Mediator of ERBB2-driven cell motility 1 (MEMO1) is an evolutionary conserved protein implicated in many biological processes; however, its primary molecular function remains unknown. MEMO1 is a highly conserved protein found in the cytosol of eukaryotic cells from yeast to humans. We conclude that MEMO1 is an iron-binding protein that modulates iron homeostasis in cancer cells. Our work reveals that the iron coordination mode in MEMO1 is very similar to that of iron-containing extradiol dioxygenases, which also display a similar structural fold.

To confirm the iron-binding site, we generated H49A and C244S mutants, along with H192A and D189N variants, because the latter residues are located in the proximity of the bound iron and were previously proposed to belong to the metal-binding site of the protein. All the mutant proteins were properly folded as shown by NMR. As shown by ITC, iron-binding affinity in the H192A and D189N mutants is not significantly changed, whereas H49A and C244S variants do not bind iron at all. Consistent with the crucial role of C244 in metal binding, no metal density was found in the C244S variant of MEMO1 crystallized in the presence of copper. Thus, metal coordination in MEMO1 is achieved by H49, H81, and C244, while H192 and D189 do not participate in metal binding in MEMO1.

>RVVCREASHAGSWYTASGPQLNAQLEGWLSQVQSTKRPARAIIAPHAGYTYCGSCAAHAYKQVDPSITRRIFILGPSHHVPLSRCALSSVDIYRTPLYDLRIDQKIYGELWKTGMFERMSLQTDEDEHSIEMHLPYTAKAMESHKDEFTIIPVLVGALSESKEQEFGKLFSKYLADPSNLFVVSSDFCHWGQRFRYSYYDESQGEIYRSIEHLDKMGMSIIEQLDPVSFSNYLKKYHNTISGRHPIGVLLNAITELQKNGMNMSFSFLNYAQSSQCRNWQDSSVSYAAGALTVH[4x]> NVIFEDEEKSKMLARLLKSSHPEDLRAANKLIKEMVQEDQKRMEKISKRVNAIEEVNNNVKLLTEMVMSHSQGGAAAGSSEDLMKEL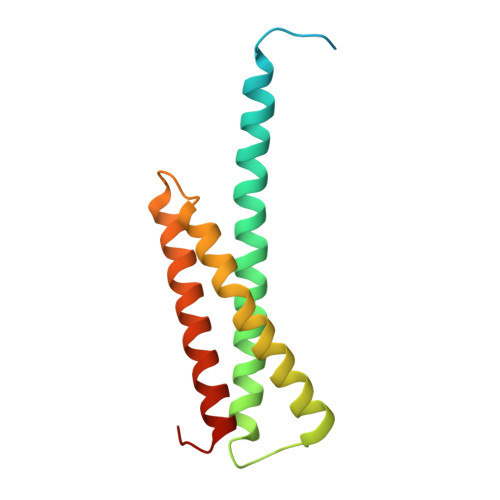YQRCERMRPTLFRLASDTEDNDEALAEILQANDNLTQVINLYKQLVRGEEVNG> GHMCQVNIKQKMQELNNEINMQQTVIYQASQALNCCVDEEHGKGSLEEAEAERLLLIATGKRTLLIDELNKLKNEGPQRKNKASPQSEFMPSKGSVTLSEIRLPLKADFVCSTVQKPDAANYYYLIILKAGAENMVATPLASTSNSLNGDALTFTTTFTLQDVSNDFEINIEVYSLVQKKDPSGL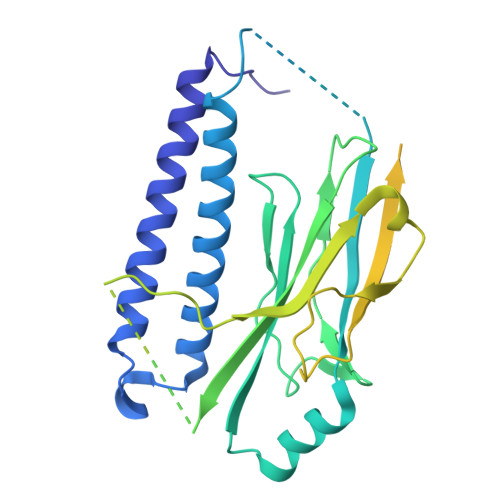DKKKKTSKSKAITPKRLLTSITTKSNIHSSVMASPGGLSAVRTSNFALVGSYTLSLSSVGNTKFVLDKVPFLSSLEGHIYLKIKCQVNSSVEERGFLTIFEDVSGFGAWHRRWCVLSGNCISYWTYPDDEKRKNPIGRINLANCTSRQIEPANREFCARRNTFELITVRPQREDDRETLVSQCRDTLCVTKNWLSADTKEERDLWMQKLNQVLVDIRLWQPDACYKPIGKP>[2x]ASMTGGQQMGRGSDSKPPYSYAQLIVQAITMAPDKQLTLNGIYTH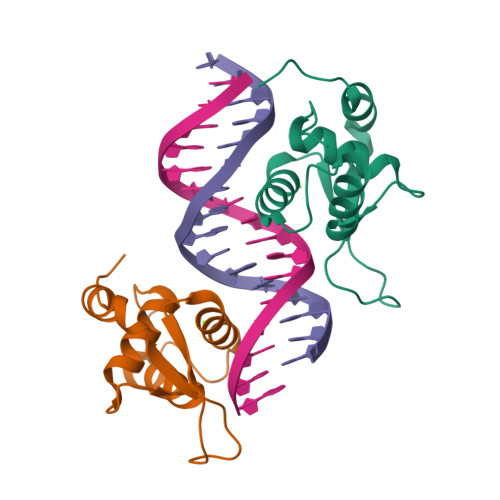ITKNYPYYRTADKGWQNSIRHNLSLNRYFIKVPRSQEEPGKGSFWRIDPASESKLIEQAFRKRRPR> PISPIETVPVKLKPGMDGPKVKQWPLTEEKIKALVEICTEMEKEGKISKIGPENPYNTPVFAIKKKDSTKWRKLVDFRELNKRTQDFWEVQLGIPHPAGLKKNKSVTVLDVGDAYFSVPLDEDFRKYTAFTIPSINNETPGIRYQYNVLPQGWKGSPAIFQSSMTKILEPFKKQNPDIVICQYMDDLYVGSDLEIGQHRTKIEELRQHLLRWGLTTPDKKHQKEPPFLWMGYELHPDKWTVQPIVLPEKDSWTVNDIQKLVGKLNWASQIYPGIKVRQLCKLLRGTKALTEVIPLTEEAELELAENREILKEPVHGVYYDPSKDLIAEIQKQGQGQWTYQIYQEPFKNLKTGKYARMRGAHTNDVKQLTEAVQKITTESIVIWGKTPKFKLPIQKETWETWWTEYWQATWIPEWEFVNTPPLVKLW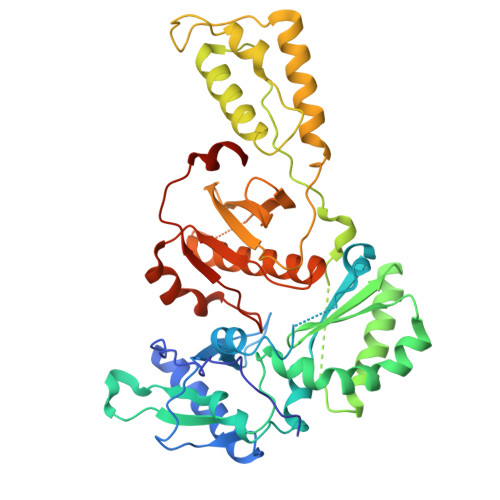YQLEKEPIVGAETF> MENLSDVFDIYAICACCKVAPTSEGTKNEPFSPRTFRGLGNKGTLPWKCNSVDMKYFRSVTTYVDESKYEKLKWKRERYLRMEASQGGGDNTSGGDNTHGGDNADKLQNVVVMGR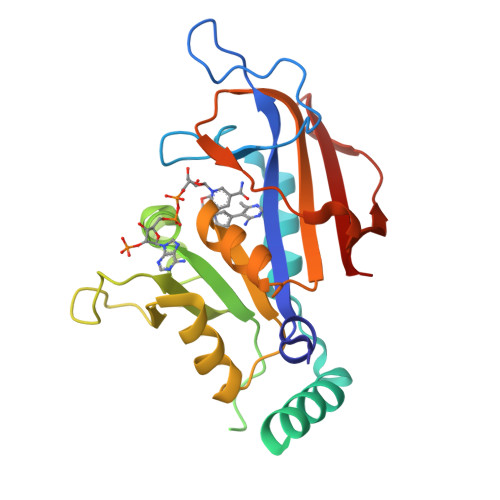SNWESIPKQYKPLPNRINVVLSKTLTKEDVKEKVFIIDSIDDLLLLLKKLKYYKCFIIGGAQVYRECLSRNLIKQIYFTRINGAYPCDVFFPEFDESEFRVTSVSEVYNSKGTTLDFLVYSKV ASPARTYL-ADENOSINE-5'-MONOPHOSPHATE 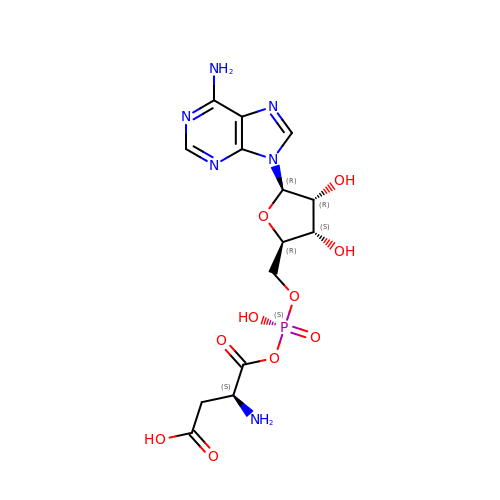| C14 H19 N6 O10 P | QPBSGQWTJLPZNF-VWJPMABRSA-N> VRATGHSYEKYNNWETIEAWTQQVATENPALISRSVIGTTFEGRAIYLLKVGKAGQNKPAIFMDCGFHAREWISPAFCQWFVREAVRTYGREIQVTELLNKLDFYVLPVLNIDGYIYTWTKSRFWRKTRSTHTG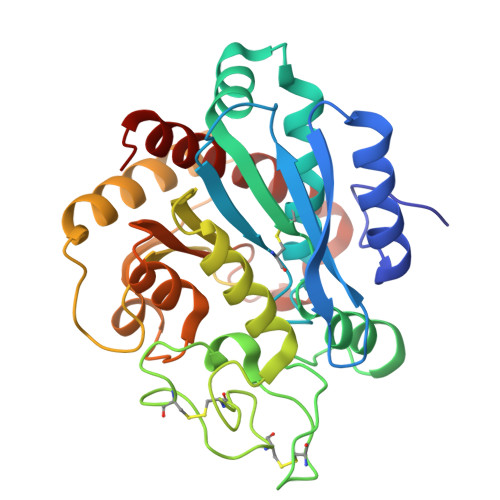SSCIGTDPNRNFDAGWCEIGASRNPCDETYCGPAAESEKETKALADFIRNKLSSIKAYLTIHSYSQMMIYPYSYAYKLGENNAELNALAKATVKELASLHGTKYTYGPGATTIYPAAGGSDDWAYDQGIRYSFTFELRDTGRYGFLLPESQIRATCEETFLAIKYVASYVLEHLY>[2x]GEEERAFLVAREELASALRRDSG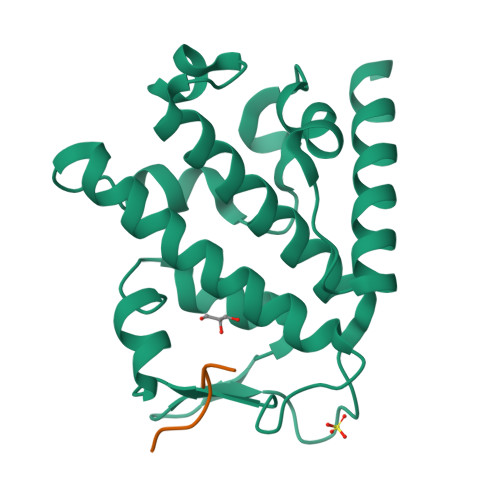QAFSLEQLRPLLASSLPLAARYLQLDAARLVRCNAHGEPRNYLNTLSTALNILEKYGRNLLSPQRPRYWRGVKFNNPVFRSTVDAVQGGRDVLRLYGYTEEQPDGLSFPEGQEEPDEHQVATVTLEVLLLRTELSLLLQNTHPRQQALEQ;>DVDLYTDS[2x]>[2x]MESTANALVVKVSYGGVLRRFRVPVKANGQLDLEMAGLKEKIAALFNLSAD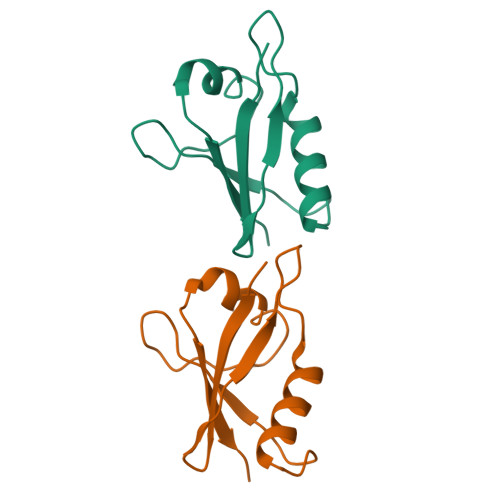AELSLTYSDEDGDVVALVDDNDLFDVTNQRLKFLKINVNAGVS> VL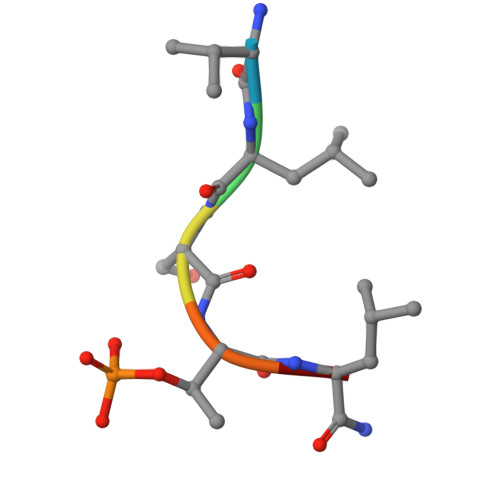STLX>[2x]AECSVDIQGNDQMQFNTNAITVDKSCKQFTVNLSHPGNLPKNVMGHNFVLSTAADMQGVVTDGMASGLDKDF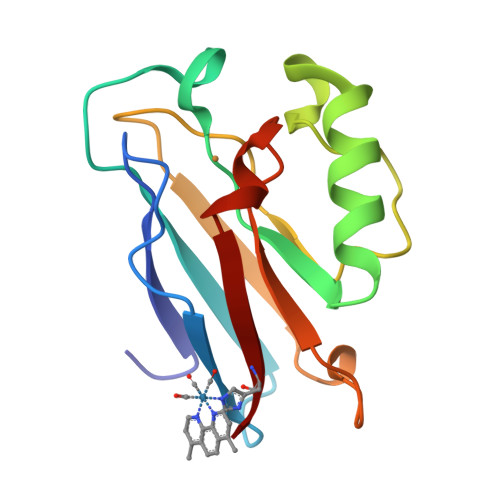LKPDDSRVIAQTKLIGSGEKDSVTFDVSKLKEGEQFMFFCTFPGHSALMFGWLHLK>[2x]GPSGAADKAGTRENQPAVVHLQGQGSAIQVKNDLSGGVLNDWSRITMNPKVFKLHPRSGELEVLVDGTYFIYSQVEVYYINFTDFASYEVVVDEKPFLQCTRSIETGKTNYNTCYTAGVCLLKARQKIAVKMVHADISINMSKHTTFFGAIRLGEAPAS;> YSNCGENEYYNQTTGLCQECPPCGPGEEPYLSCGYGTKDEDYGCVP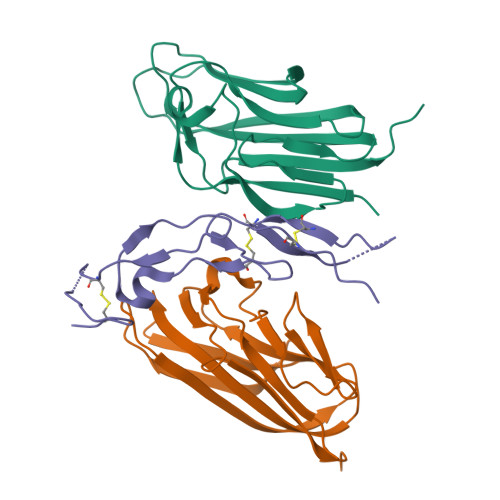CPAEKFSKGGYQICRRHKDCEGFFRATVLTPGDMENDAECGPCLPGYYMLENRPRNIYGMVCYSCLLAPPNTKECVG2-hydroxybenzonitrile | C7 H5 N O | 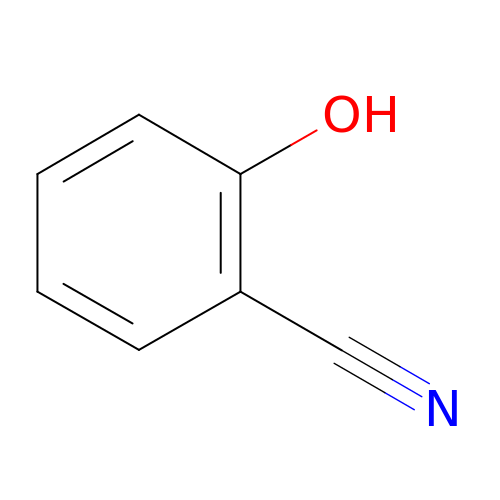CHZCERSEMVWNHL-UHFFFAOYSA-N>[3x]GSHMLEMRIGHGFDVHAFGGEGPIIIGGVRIPYEKGLLAHSDGDVALHALTDALLGAAALGDIGKLFPDTDPAFKGADSREL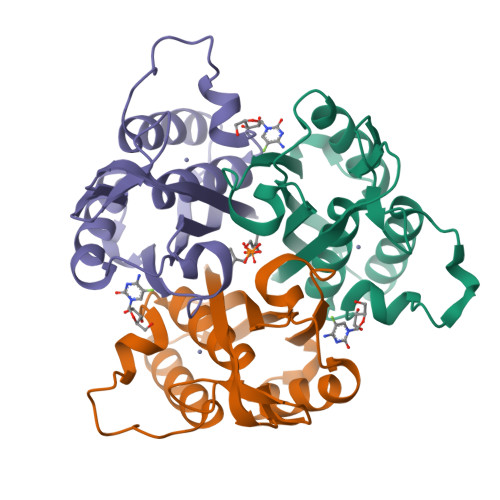LREAWRRIQAKGYTLGNVDVTIIAQAPKMLPHIPQMRVFIAEDLGCHMDDVNVKATTTEKLGFTGRGEGIACEAVALLIKATK> ALQQLFENNVRWAEAIKQEDPDFFAKLARQQTPEYLWIGCSDARVPANEIVGMLPGDL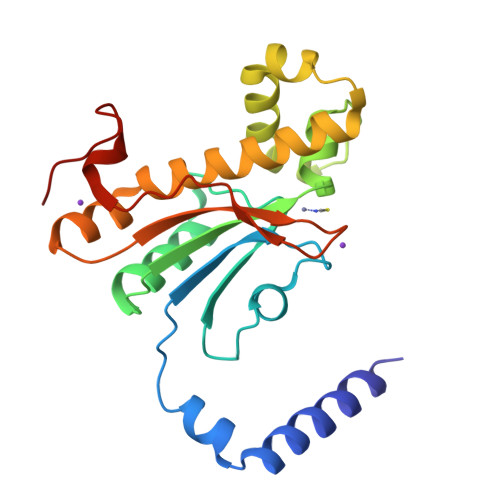FVHRNVANVVLHTDLNCLSVIQFAVDVLKVKHILVTGHYGCGGVRASLHNDQLGLIDGWLRSIRDLAYEYREHLEQLPTEEERVDRLCELNVIQQVANVSHTSIVQNAWHRGQSLSVHGCIYGIKDGLWKNLNVTVSGLDQLPPQYRLSPL> QEGTSPMQKETRFLPGTNVEYEDYSTFFDKFSASGGFVLFNSNRKKYTIYNRKESTSRFAPASTYKVFSALLALESGIITKNDSHMTWDGTQYPYKEWNQDQDLFSAMSSSTTWYFQKLDRQIGEDHLRHYLKSIHYGNEDFSVPADYWLDGSLQISPLEQVNILKKFYDNEFDFKQSNIETVKDSIRLEESNGRVLSGKTGTSVINGELHAGW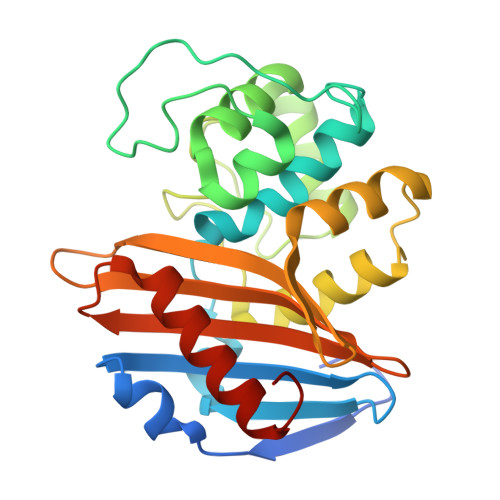FIGYVETADNTFFFAVHIQGEKRAAGSSAAEIALSILDKKGIYPSVSR4-acetamido-3-fluoranyl-~{N}-(4-oxidanylcyclohexyl)-5-[(1~{S})-1-phenylethoxy]benzamide 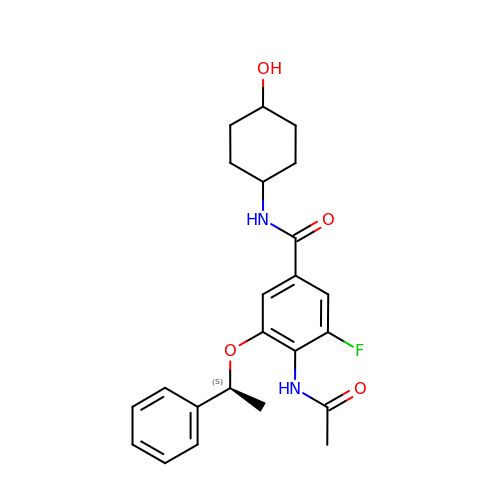| C23 H27 F N2 O4 | FRBRZGLUFOZRGD-JVPBZIDWSA-N>SNATTSQPVQLKIASYGLLKNLTWVSLENQVPGVGEVKVQIQAVPVNFRDILNALGMLQEHNQTKLGITSVDHLTFGFEAVGVIVGVGLGVSQWQIGDEVMVIGCHDAFSSFIICSPNNLVAKPANLKLIEAATIPIPFFTAYHGLYNLAKIQSGERVLIHAASGGTGQAAIQLAQFWGAEVFATTSPQKMAVLREQGIKHVMNSRTTEFANEIRELTQGKGVDVIFNSLTHGEYIQKNLDVLALEGRYIEISKRKIWSHSQVAQKRSDIKYFPFDLLEEFNRDNQLYYQIWKKLIQCFENKE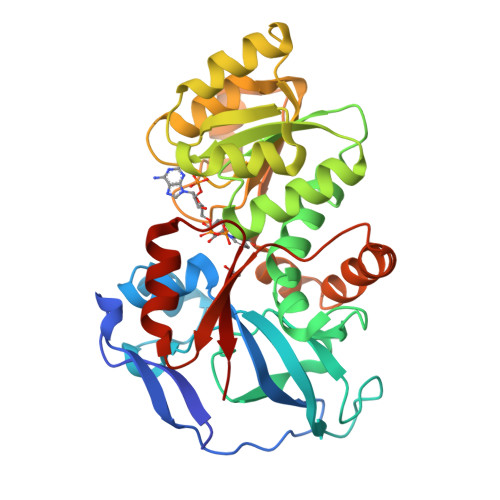LHPLVYKTFPNEDIVEAFRYLQRSKHIGRVVVTMP[3x]>QFMEGNGPAAVHYQPASPPRDACVYSSCYSEENVWKLCEYIKNHDQYPLEECYAVFISNERKMIPIWKQQARPGDGPVIWDYHVVLLHVSSGGQSFIYDLDTVLPFPCLFDTYVEDAIKSDDDIHPQ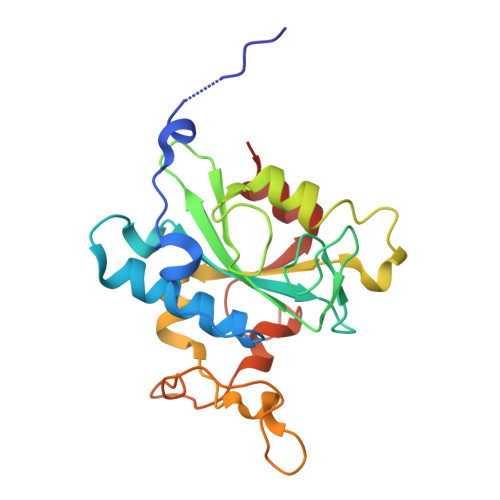FRRKFRVICADSYLKNFASDRSHMKDSSGNWREPPPPYPCIETGDSKMNLNDFISMDPKVGWGAVYTLSEFTHRFGS[2x]>AVREYQKKRRRERIFRAAMELFRNRGFQETTATEIAKAAHVSRGTFFNYYPYKEAVLLDYGSQLLAGLREEVRRLLAQGREPVEVLRHLFRVLAEGTAREKDLLLPMFYELLNPDPVRARAAFEALPLGDLIAEILKPLREQGVLRQDFSLERMGRTLADLYFLSALRWAAYTPGRDLAEELE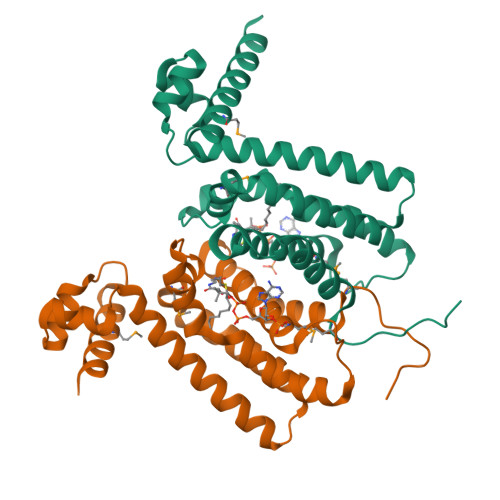KNLRLLLEGMLVREAPAPGGL[4x]> VTSITLDLVNPTAGQYSSFVDKIRNNVKDPNLKYGGTDIAVIGPPSKEKFLRINFQSSRGTVSLGLKRDNLYVVAYLAMDNTNVNRAYYFKSEITSAELTALFPEATTANQKALEYTEDYQSIEKNAQITQGDKSRKELGLGIDLLLTFMEAVNKKARVVKNEARFLLIAIQMTAEVARFRYIQNLVTKNFPNKFDSDNKVIQFEVSW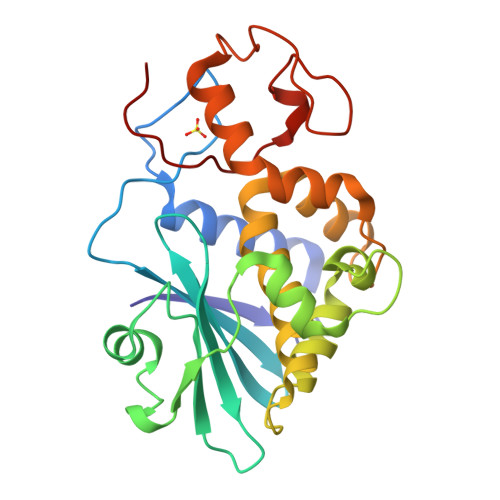RKISTAIYGDAKNGVFNKDYDFGFGKVRQVKDLQMGLLMYLGKPK> GLNDFQKQKIKFTFDFFLDMNHDGSIQDNDFEDMMTRYKEVNKGSLSDADYKSMQASLEDEWRDLKGRADINKDDVVSWEEYLAMWEKTIATCKSVA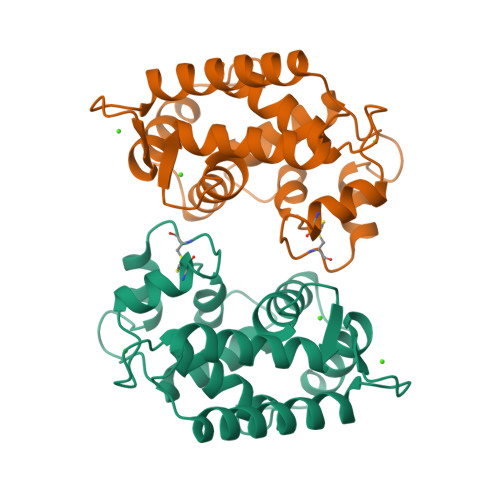DLPAWCQNRIPFLFKGMDVSGDGIVDLEEFQNYCKNFQLQCADVPAVYNVITDGGKVTFDLNRYKELYYRLLTSPAADAGNTLMGQKP> QGFSLAQYLQEQKTIVETALDQSLVITEPVTIYEAMRYSLLAGGKRLRPILCLAACEMLGGTAAMAMNTACALEMIHTMSLIHDDLPAMDNDDLRRGKPTNHKVYGEDIAILAGDALLSYAFEYVARTPDVPAERLLQVIVRLGQAVG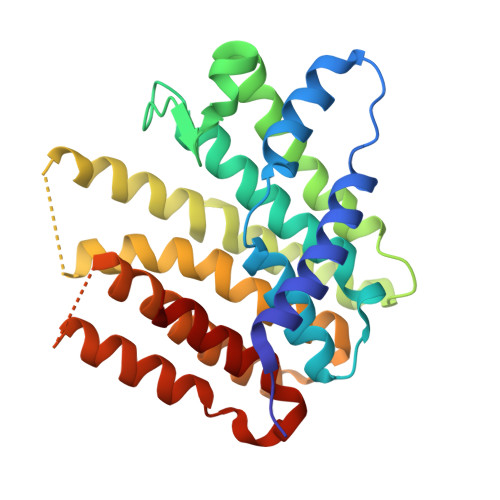AEGLVGGQVVDLESEGKETLNFIHTHKTGALLEVCVTAGAILAGAKPEEVQLLSRYAQNIGLAFQIVDDSQAEAQKLVAEAIASLEPYGEKANPLKALAEYIVNR> MSSVTWAPGNYPSTRRSDHVDTYQSASKGEVPVPDPYQWLEESTDEVDKWTTAQADLAQSYLDQNADIQKLAEKFRASRNYAKFSAPTLLDDGHWYWFYNRGLQSQSVLYRSKEPALPDFSKGDDNVGDVFFDPNVLAADGSAGMVLCKFSPDGKFFAYAVSHLGGDYSTIYVRSTSSPLSQASVAQGVDGRLSDEVKWFKFSTIIWTKDSKGFLYQRYPARERHEGTRSDRNAMMCYHKVGTTQEEDIIVYQDNEHPEWIYGADTSEDGKYLYLYQFKDTSKKNLLWVAELDEDGVKSGIHWRKVVNEYAADYNIITNHGSLVYIKTNLNAPQYKVITIDLSKDEPEIRDFIPEEKDAKLAQVNCANEEYFVAIYKRNVKDEIYLYSKAGVQLTRLAPDFVGAASIANRQKQTHFFLTLSGFNTPGTIARYDFTAPETQRFSILRTTKVNELDPDDFESTQVWYESKDGTKIPMFIVRHKSTKFDGTAAAIQYGYGGFATSADPFFSPIILTFLQTYGAIFAVPSIRGGGEFGEEWHKGGRRETKVNTFDDFIAAAQFLVKNKYAAPGKVAINGAANGGLLVMGSIVRAPEGTFGAAVPEGGVADLLKFHKFTGGQAWISEYGNPSIPEEFD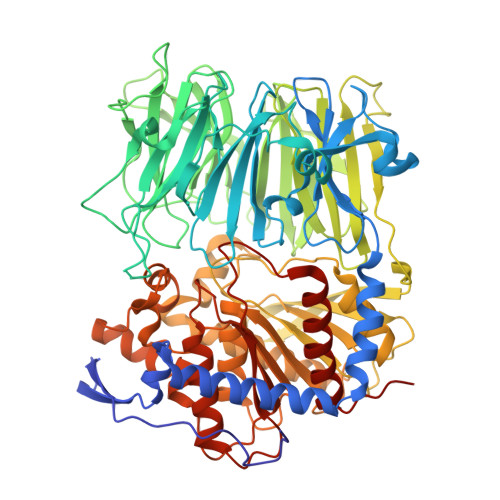YIYPLSPVHNVRTDKVMPATLITVNIGDGRVVPMHSFKFIATLQHNVPQNPHPLLIKIDKSWLGHGMGKPTDKNVKDAADKWGFIARALGLELKTVE>[5x]GQ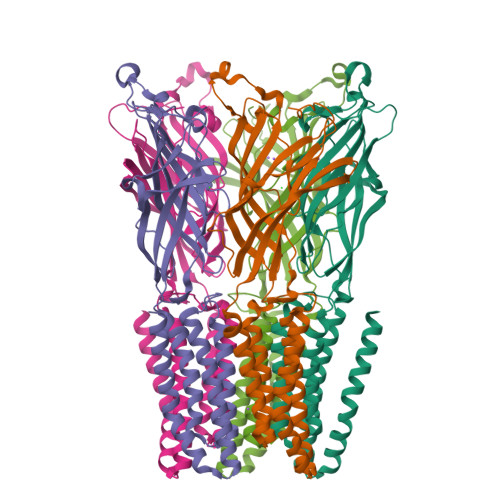DMVSPPPPIADEPLTVNTGIYLIESYSLDDKAETFKVNAFLSLSWKDRRLAFDPVRSGVRVKTYEPEAIWIPEIRFVNVENARDADVVDISVSPDGTVQYLERFSARVLSPLDFRRYPFDSQTLHIYLIVRSVDTRNIVLAVDLEKVGKNDDVFLTGWDIESFTAVVKPANFALEDRLESKLDYQLRISRQYFSFIPNIILPMLFILFISWTAFWSTSYEANVTLVVSTLIAHIAFNILVETNLPKTCYMTYTGAIIFMIYLFYFVAVIEVTVQHYLKVESQPARAASITRASRIAFPVVFLLANIILAFLFFGF Nucleoside diphosphate kinases (NDPKs) catalyze the reversible transfer of the phosphoryl γ of nucleoside triphosphates to nucleoside diphosphates. The two-step reaction proceeds via a covalent intermediate, the enzyme being transiently phosphorylated on a conserved histidine residue, His117 in Mycobacterium tuberculosis NDPK (Mt-NDPK). Crystal structure of the Mt-NDPK has been solved. It is a hexamer with a tertiary and quaternary structure very similar to other hexameric NDPKs.

One interaction present in Mt-NDPK but missing in other NDPKs, is the intersubunit salt bridge Arg80-Asp93 located on the protein surface. Here, to elucidate the crucial role of that salt bridge for hexamer and overall protein stability, a mutant having the salt bridge abolished (D93N) has been prepared. The D93N mutant crystallizes along two different space groups. The two structures are similar (0.40 Å of rmsd for 135 Cα) and differ only slightly in the conformation of αA and α2 helices due to crystal contacts. The overall B-factor values of the two D93N structures (64 Å2 and 71 Å2) are similar and higher than that of the wild type (31 Å2). Analysis of B-factor reveals that (1) two domains, the αA-α2 region (40–70) and the CTerm part (120–136), are highly flexible and (2) the beginning of the Kpn-loop where the mutation is located appears more flexible in the mutant than in the WT structure. The D93N mutant enzymes displayed catalytic properties very similar to those of the wt enzyme, within experimental errors. In presence of urea, the mutation of the negatively charged Asp93 into the neutral Asn had a dramatic effect on the hexamer stability. : the c1/2 of the wt hexamer decreased from 5.2 M to less than 0.5 M for the D93N mutant. The D93N mutation appears to decrease the protein stability because the negative charge of the Asp93 interacts with distant protein charges and stabilizes the hexamer. The lower contact surfaces between subunits, as compared to other NDPKs, are compensated by the intersubunit salt bridge Arg80-Asp93.

>MTERTLVLIKPDGIERQLIGEIISRIERKGLTIAALQLRTVSAELASQHYAEHEGKPFFGSLLEFITSGPVVAAIVEGTRAIAAVRQLAGGTNPVQAAAPGTIRGDFALETQFNLVHGSDSAESAQREIALWFPGA[2x]> MEGLTIDLKNFRKPGEKTFTQRSRLFVGNLPPDITEEEMRKLFEKYGKAGEVFIHKDKGFGFIRLETRTLAEIAKVELDNMPLRGKQL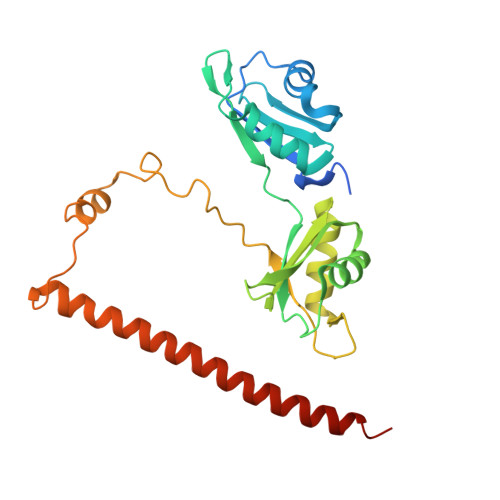RVRFACHSASLTVRNLPQYVSNELLEEAFSVFGQVERAVVIVDDRGRPSGKGIVEFSGKPAARKALDRCSEGSFLLTTFPRPVTVEPMDQLDDEEGLPEKLVIKNQQFHKEREQPPRFAQPGSFEYEYAMRWKALIEMEKQQQDQVDRNIKEAREKLEMEMEAARHEHQVMLM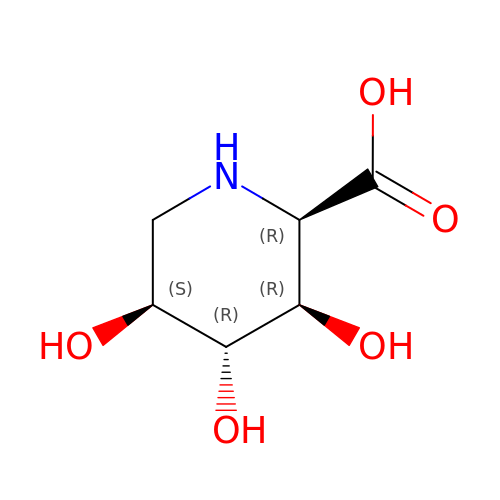(2R,3R,4R,5S)-3,4,5-trihydroxypiperidine-2-carboxylic acid | C6 H11 N O5 | ZHFMVVUVCALAMY-NRXMZTRTSA-N>[18x]MFVDDVTRAFESGDFARPNLFQVEISYLGQNFTFQCKATALPAGIVEKIPVGFMNRKINVAGDRTFDDWTVTVMND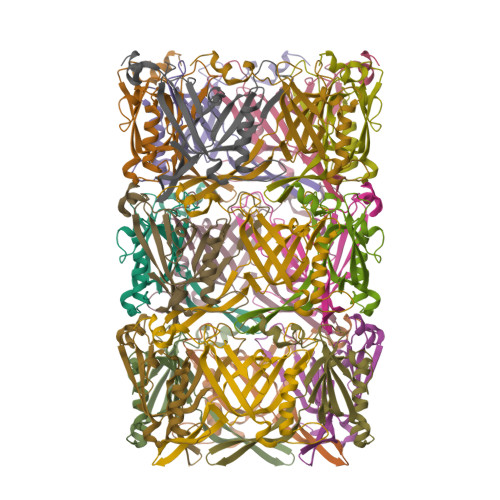EAHDARQKFVDWQSIAAGQGNEITGGKPAEYKKSAIVRQYARDAKTVTKEIEIKGLWPTNVGELQLDWDSNNEIQTFEVTLALDYWE>ADLPGSHDLDILPRFPRAEIVDFRQAPSEERIYPLGAISRISGRLRMEGEVRAEGELTALTYRLPPEHSSQEAFAAARTALLKADATPLFWCERRDCGSSSLLANAVFGNAKLYGPDEQQAYLLVRLAAPQENSLVAVYSITRGNRRAYLQAEELKADAPLAELLPSPATLLRLLKANGELTLSHVPAEPAGSWLEL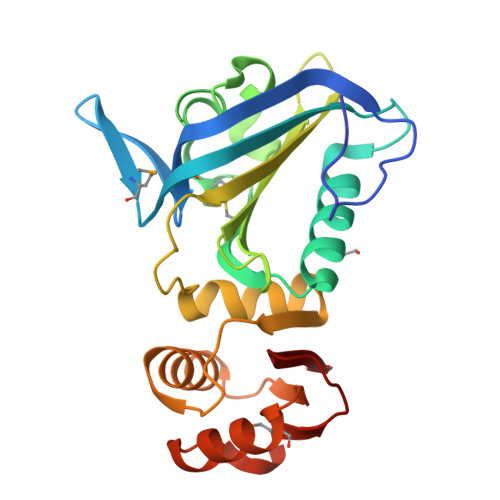LVRTLRLDTGVRVELSGKHAQEWRDALRGQGVLNSRMELGQSEVEGLHLNWLR[2x]>[2x]HHHHHHGTVIGHRDGYGFLRVEGRKDDLYLSSEQMKTCIHGDQVLAQPLGVDRKGRREARIVRVLVPKTSQIVGRYFTEAGVGFVVPDDSRLSFDIL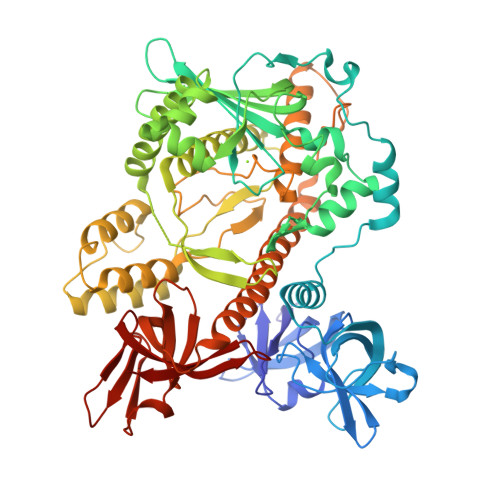IPPDQIMGARMGFVVVVELTQRPTRRTKAVGKIVEVLGDNMGTGMAVDIALRTHEIPYIWPQAVEQQVAGLKEEVPEEAKAGRVDLRDLPLVTIDGEDARDFDDAVYCEKKRGGGWRLWVAIADVSYYVRPSTPLDREARNRGTSVYFPSQVIPMLPEVLSNGLCSLNPQVDRLCMVCEMTVSSKGRLTGYKFYEAVMSSHARLTYTKVWHILQGDQDLREQYAPLVKHLEELHNLYKVLDKAREERGGISFESEEAKFIFNAERRIERIEQTQRNDAHKLIEECMILANISAARFVEKAKEPALFRIHDKPSTEAITSFRSVLAELGLELPGGNKPEPRDYAELLESVADRPDAEMLQTMLLRSMKQAIYDPENRGHFGLALQSYAHFTSPIRRYPDLTLHRAIKYLLAKEQGHQGNTTETGGYHYSMEEMLQLGQHCSMAERRADEATRDVADWLKCDFMLDQVGNVFKGVISSVTGFGFFVRLDDLFIDGLVHVSSLDNDYYRFDQVGQRLMGESSGQTYRLGDRVEVRVEAVNMDERKIDFSLI> APSFDCGKPQVEPKKCPGRVVGGCVAHPHSWPWQVSLRTRFGMHFCGGTLISPEWVLTA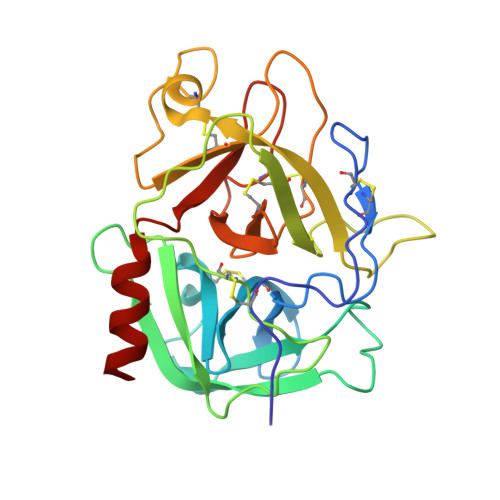AHCLEKSPRPSSYKVILGAHQEVNLEPHVQEIEVSRLFLEPTRKDIALLKLSSPAVITDKVIPACLPSPNYVVADRTECFITGWGETQGTFGAGLLKEAQLPVIENKVCNRYEFLNGRVQSTELCAGHLAGGTDSCQGDAGGPLVCFEKDKYILQGVTSWGLGCARPNKPGVYVRVSRFVTWIEGVMRNN> GAMGSGLAKYLPGATNLLSKSGEVSLGSLVGKTVFLYFSASWCPPCRGFTPVLAEFYEKHHVAKNFEVVLISWDENESDFHDYYGKMPWLALPFDQRSTVSELGKTFGVESIPTLITINADTGAIIGTQARTRVIEDPDGANFPW;>GAMGSGLAKYLPGATNLLSKSGEVSLGSLVGKTVFLYFSASWCPPCRGFTPVLAEFYEKHH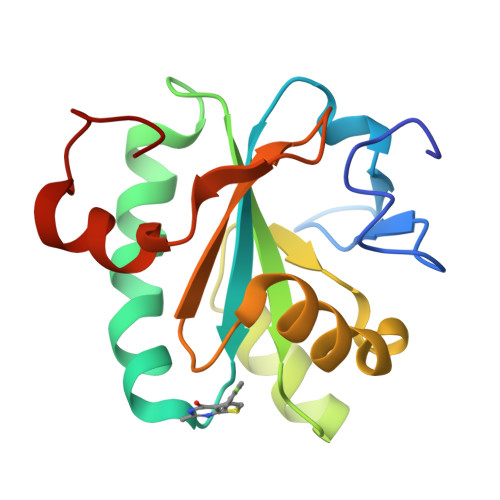VAKNFEVVLISWDENESDFHDYYGKMPWLALPFDQRSTVSELGKTFGVESIPTLITINADTGAIIGTQARTRVIEDPDGANFPWPN[2x]>[3x]MASMTGGQQMGRGSMAGVLPAHGTQHGIRLPLRSGLGGAPLGLRLPRETDEEPEEPGRRGSFVEMVDNLRGKSGQGYYVEMTVGSPPQTLNILVDTGSSNFAVGAAPHPFLHRYYQRQLSSTYRDLRKGVYVPYTQGKWEGELGTDLVSIPHGPNVTVRANIAAITESDKFFINGSNWEGILGLAYAEIARPDDSLEPFFDSLVKQTHVPNLFSL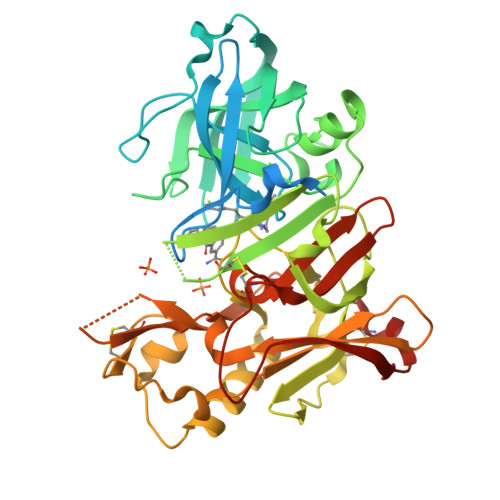QLCGAGFPLNQSEVLASVGGSMIIGGIDHSLYTGSLWYTPIRREWYYEVIIVRVEINGQDLKMDCKEYNYDKSIVDSGTTNLRLPKKVFEAAVKSIKAASSTEKFPDGFWLGEQLVCWQAGTTPWNIFPVISLYLMGEVTNQSFRITILPQQYLRPVEDVATSQDDCYKFAISQSSTGTVMGAVIMEGFYVVFDRARKRIGFAVSACHVHDEFRTAAVEGPFVTLDMEDCGYNIPQTDES(2~{R})-2-(4-bromanylphenoxy)propanamide | C9 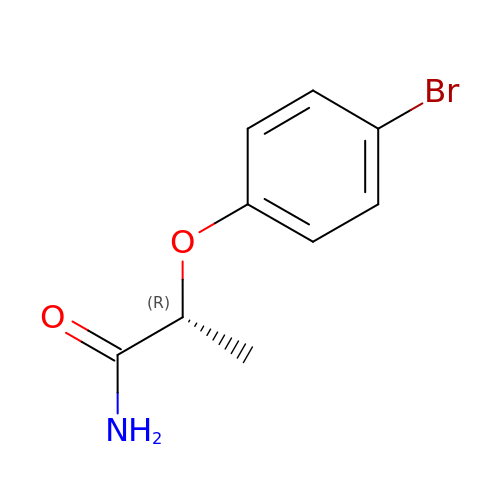H10 Br N O2 | GBEDJWZQBGSKBM-ZCFIWIBFSA-N>[2x]GPGSMQLSFQDRTYLVTGGGSGIGKGVAAGLVAAGASVMIVGRNPDKLAGAVQELEALGANGGAIRYEPTDITNEDETARAVDAVTAWHGRLHGVVHCAGGSENIGPITQVDSEAWRRTVDLNVNGTMYVLKHAAREMVRGGGGSFVG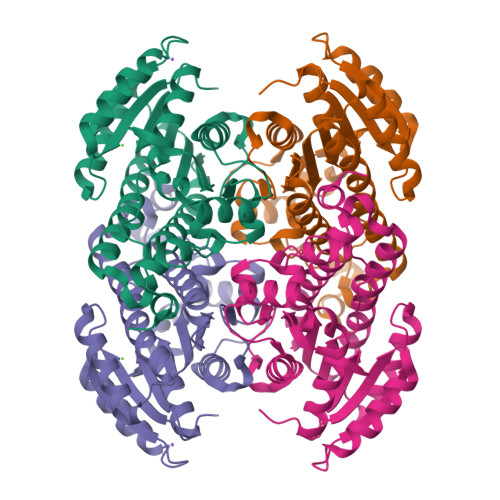ISSIAASNTHRWFGAYGVTKSAVDHLMQLAADELGASWVRVNSIRPGLIRTDLVAAITESAELSSDYAMCTPLPRQGEVEDVANMAMFLLSDAASFVTGQVINVDGGQMLRRGPDFSAMLEPVFGRDALRGLV> GSSHHHHHHSGDPASMNNHPEVKIKTILSLFLNINI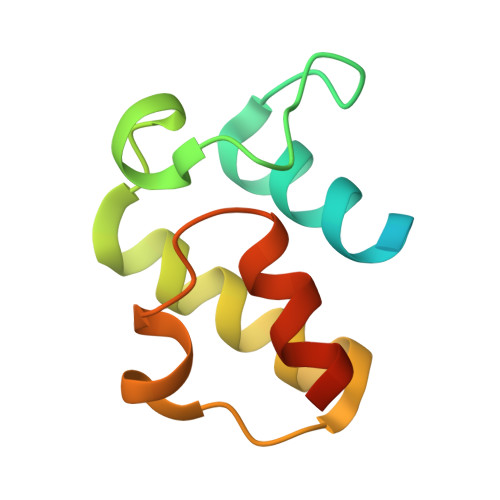DDFNMDANLADAYDMDSTELADLAKEIEKEFGISVTKSQFSHWETGRAVLDFVSSSLNDKN>[6x]SMEDVEETYIMVKPDGIQRGLVGEIISRFEKKGFKLIGLKMFQCPKELAEEHYKDLSAKSFFPNLIEYITSGPVVCMAWEGVGVVASARKLIGKTDPLQAEPGTIRGDLAVQTGRNIVHGSD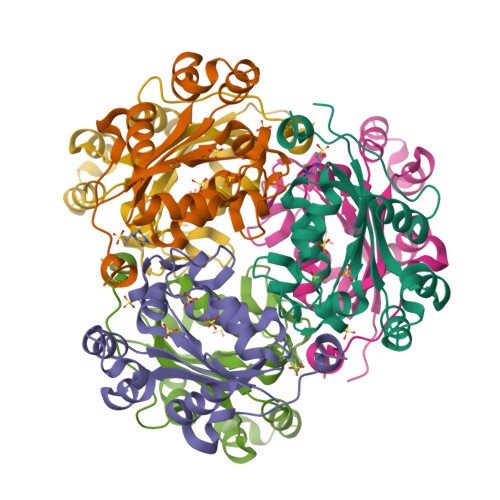SPENGKREIGLWFKEGELCKWDSALATWLRE Poxviruses are a group of enveloped viruses, the entry of which require the fusion between viral envelop and cell membrane. In poxviruses, however, its fusion process is mediated by a large proteinaceous machinery, which is designated as the entry-fusion complex (EFC). It is believed that poxvirus EFC is composed of at least eleven virus-encoded protein subunits, among which the A16 and G9 subunits (nomenclatures of A16, G9 and other proteins refer to vaccinia virus, a prototype membrane of Orthopoxvirus genus in Poxviridae family) form a sub-complex and play a key role in EFC assembly and function. In this study, we reported the crystal structure of the A16/G9 sub-complex from the vaccinia virus.

The final structure, with a resolution of 2.7-Å, was refined to Rwork = 0.243 and Rfree = 0.273, respectively. Within the crystallographic asymmetric unit of the structure, a single A16 protein and one G9 protein are present in a 1:1 binding mode. Traceable electron densities can be observed for A16 residues L7-C291 and G9 amino acids E8-N268. Both A16 and G9 feature with an extended rod-like fold. Sterically, the NTD and CTD of A16 are linked via a relatively long loop, which might be of certain flexibility. Unlike that of A16, however, the inter-domain linker in G9 is of short length and an inter-domain disulfide-bond (C89/C127) is observed to form, dragging the two domains into close proximity. Resultantly, the two protein subunits are aligned almost in parallel, leading to good complementarity and the formation of an extended binding interface. In order to characterize the atomic binding details between the two proteins, we further subdivided the binding interface into five patches (Patch1-Patch5) based on the G9 components involved in A16-engagement. Within these three patches, a large number of interface residues are identified for inter-molecule contacts, including G9-residues F92-N93 and T95-H96, and A16-residues D170, T173, R177, K194-P195, S198, D202 and F227 in Patch3, G9-residues D120-H122, R142-N143, H146-Q147, G150-S151, N154, H191-H192, A195 and N197, and A16-residues E166, R193-K194, S198, S201, D223-F227, D229-T230, Y233-V234, Y282-N283 and R290 in Patch4 and G9-residues C243, C248-A251, V253, Y261, L264-G265 and C267-N268, and A16-residues D257-K258, L260-R263, C265-W266, Q287 and C291 in Patch5. It is noteworthy that the amino acids involved in vaccinia virus A16/G9 binding are highly conserved among members of the Orthopoxvirus genus, demonstrating that the orthopoxviruses, including the monkeypox virus, would share quite similar binding patterns and likely the same interaction details for A16/G9 sub-complex formation.

> MGAAVTLNRIKIAPGIADIRDKYMELGFNYPEYNRAVKFAEESYTYYYETSPGEIKPKFCLIDGMSIDHCSSFIVPEFAKQYVLIHGEPCSSFKFRPGSLIYYQNEVTPEYIKDLKHATDYIASGQRCHFIKKDYLLGDSDSVAKCCSKTNTKHCPKIFNNNYKTEHCDDFMTGFCRNDPGNPNCLEWLRAKRKPAMSTYSDICSKHMDARYCSEFIRIIRPDYFTFGDTALYVFCNDHKGNRNCWCANYPKSNSGDKYLGPRVCWLHECTDESRDRKWLYYNQDVQRTRCKYVGCTINVNSLALKNSQAELTSNCTRTTSAVGDVHPGEPVVKDKIKLPTWHHHHHH;> MGGGVSVELPKRDPPPGVPTDEMLLNVDKMHDVIAPAKLLEYVHIGPLAKDKEDKVKKRYPEFRLVNTGPGGLSALLRQSYNGTAPNCCRTFNRTHYWKKDGKISDKYEEGAVLESCWPDVHDTGKCDVDLFDWCQGDTFDRNICHQWIGSAFNRSNRTVEGQQSLINLYNKMQTLCSKDASVPICESFLHHLRAHNTEDSKEMIDYILRQQSADFKQKYMRCSYPTRDKLEESLKYAEPRECWDPECSNANVNFLLTRNYNNLGLCNIVRCNTSVNNLQMDKTSSLRLSCGLSNSDRFSTVPVNRAKVVQHNIKHSFDWSHPQFEK> QDWLTFQKKHITNT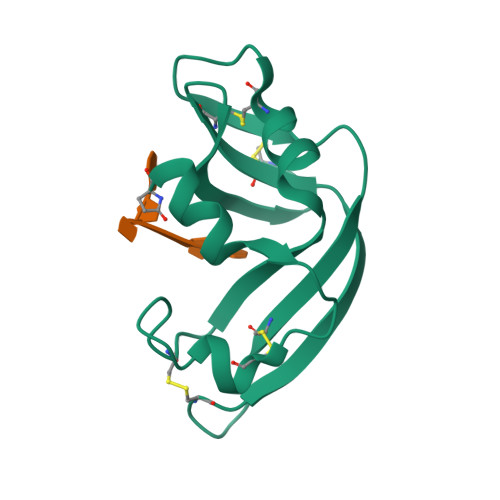RDVDCDNIMSTNLFHCKDKNTFIYSRPEPVKAICKGIIASKNVLTTSEFYLSDCNVTSRPCKYKLKKSTNKFCVTCENQAPVHFVGVGSC5-[(E)-(5-CHLORO-2-OXO-1,2-DIHYDRO-3H-INDOL-3-YLIDENE)METHYL]-N-[2-(DIETHYLAMINO)ETHYL]-2,4-DIMETHYL-1H-PYRROLE-3-CARBOXAMIDE | C22 H27 Cl N4 O2 | 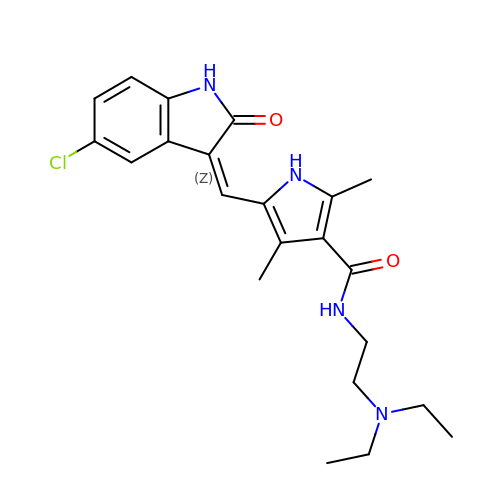XPLJEFSRINKZLC-ATVHPVEESA-N> SNAMAKFNVENEHVEVEIEKLYKFSPELVYEAWTKKDLLKQWFMTSARTNKEIEADVKEGGKYRIVDQQRN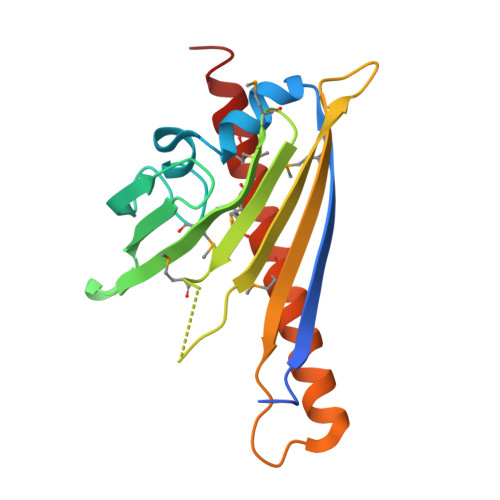GKVNVIEGIYESLVMDEYVKMTIGMPGLSETQDVIEVEFFERETGGTQMLFYYRSLVEKERRFTNLEYKQKKKEYHDAMVHGFELMFDKMYHVIETSTQQ>[2x]MPGEIRPTIGQQMETGDQRFGDLVFRQLAPNVWQHTSYLDMPGFGAVASNGLIVRDGGRVLVVDTAW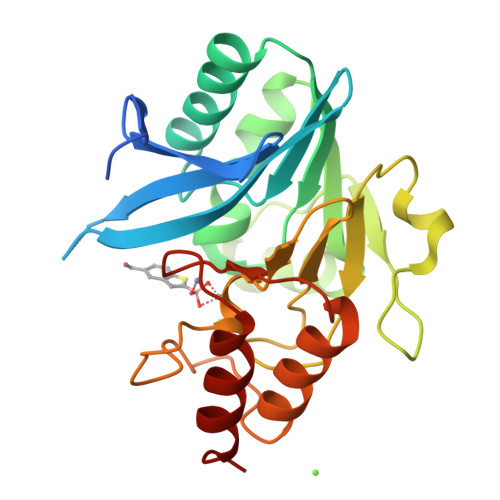TDDQTAQILNWIKQEINLPVALAVVTHAHQDKMGGMDALHAAGIATYANALSNQLAPQEGMVAAQHSLTFAANGWVEPATAPNFGPLKVFYPGPGHTSDNITVGIDGTDIAFGGCLIKDSKAKSLGNLGDADTEHYAASARAFGAAFPKASMIVMSHSAPDSRAAITHTARMADKLR Macrophage infectivity potentiator (MIP) proteins are key microbial virulence factors that facilitate host cell infection, intracellular pathogen replication, and dissemination. They are found in a variety of pathogens of both bacterial and eukaryotic origin, including Burkholderia pseudomallei, the causative agent of melioidosis, Legionella pneumophila, leading to Legionnaires’ disease, and the protozoan parasites Trypanosoma cruzi and Leishmania subspecies. All MIP proteins share a peptidyl-prolyl-cis–trans-isomerase (PPIase) domain resembling the FK506 binding protein domains of human FKBPs. All MIP and FKBP proteins share a general domain topology in their core PPIase domain with an amphipathic five-stranded β-sheet wrapping around a short α-helix, thereby forming a hydrophobic active site32. Inhibition of secreted MIP proteins diminishes macrophage invasion and leads to the reduction of overall pathogen load and virulence, as shown for L. pneumophila and B. pseudomallei, respectively.

Here, we determined the crystal structures of B. pseudomallei MIP (BpMIP), which contains only the core PPIase domain and T. cruzi MIP (TcMIP), which features the PPIase domain and a free-standing α-helix (“stalk”), in complex with fluorinated pipecolic acid inhibitors. In all cases, we found that the inhibitor molecules bound within the expected FKBP-like domain cleft that forms the MIP active site. NJS224 carries a fluorinated thioaryl group (henceforth denoted X1) and an isopropyl group (X2A) and gives rise to a single resonance at −113.19 ppm. The spectrum of NJS227, which carries the same X1 moiety in addition to a para-fluorobenzyl group (X2B), features two 19F resonances. In agreement with very similar KD values for either ligand, the distinguishing moieties, i.e., the iso-propyl group in NJS224 and the para-fluorobenzyl moiety in NJS227, do not make substantial protein contacts and furthermore face in opposite directions. Comparing the crystal structures of TcMIP and BpMIP with NJS227, the inhibitor adopts a highly similar binding stance and the respective protein side chains align well (RMSD = 0.58 Å). The fluorobenzyl group attached to the sulfoxyl group, i.e., the group present in either inhibitor, is nestled into a hydrophobic pocket formed by F43 in β-strand 3a and V97/I98 in the loop between β4 and β5 in BpMIP and the corresponding residues F73 and M125/I126 in TcMIP. In the crystal structures, the inhibitor’s piperidine ring rests within a hydrophobic cage formed by conserved aromatic residues (Y33/Y63, F53/F85, and W66/W94 in BpMIP and TcMIP, respectively). Interestingly, for BpMIP, the NJS224 X1 line width is broader, while for TcMIP, NJS227 displays broader lines and thus presumably reduced flexibility. Finally, it needs to be noted that for both TcMIP and BpMIP, the X2B19F resonance showed a much more pronounced CSP than the X1 moiety.

>DAASHEERMNNYRKRVGRLFMEQKAAQPDAVKLPSGLVFQRIARGSGKRAPAIDDKCEVHYTGRLRDGTVFDSSRERGKPTTFRPNEVIKGWTEALQLMREGDRWRLFIPYDLAYGVTGGGGMIPPYSPLEFDVELISIKDGGKGRTAEEVDEILRKAEED[2x]> QMNYEEVIKKYRGEENFDHAAYDWRLHSGVTPVKDQKNCGSCWAFSSIGSVESQYAIRKNKLITLSEQELVDCSFKNYGCNGGLINNAFEDMIELGG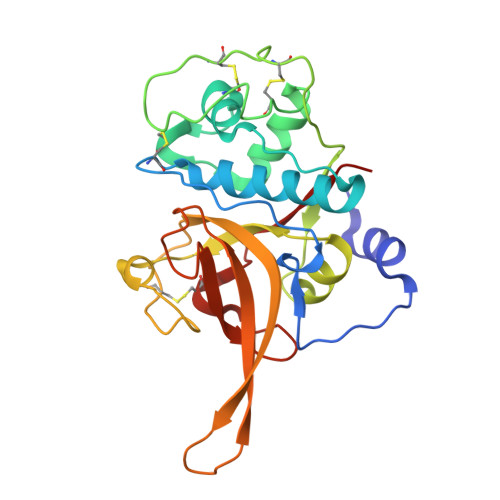ICPDGDYPYVSDAPNLCNIDRCTEKYGIKNYLSVPDNKLKEALRFLGPISISVAVSDDFAFYKEGIFDGECGDQLNHAVMLVGFGMKEIVNPLTKKGEKHYYYIIKNSWGQQWGERGFINIETDESGLMRKCGLGTDAFIPLIE~{N}-(2-morpholin-4-ylethyl)-2-sulfanyl-benzamide | C13 H18 N2 O2 S | 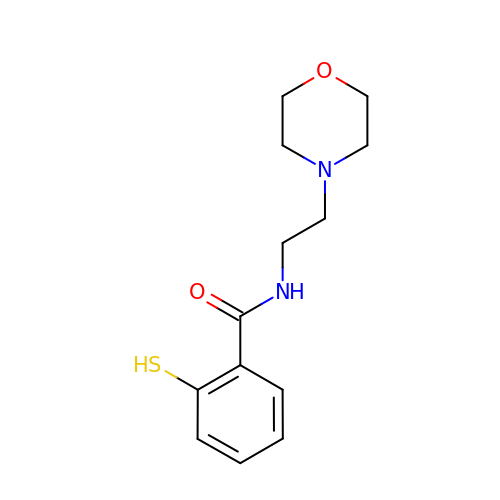ZLDHBHAHQHKIKU-UHFFFAOYSA-N4-(2-HYDROXYPHENYLSULFINYL)-BUTYLPHOSPHONIC ACID | C10 H15 O5 P S | 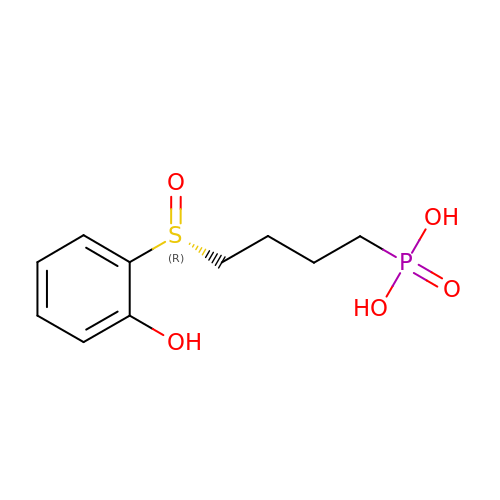FFIGWLBWBXCVHW-QGZVFWFLSA-N>[2x]MGSSHHHHHHSSGLVPRSHMSPDLTYTEVNQNLAARENASWFSPVRFAYDW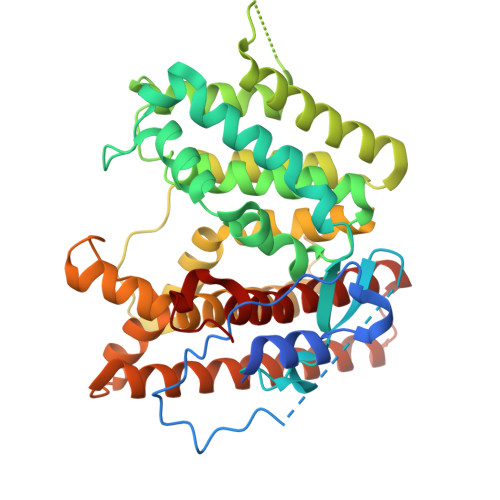LEDAPIEHLTAVPLKIRTDSPLASPKPSNVKEQSITENNENSFSISPQLTGLPWPTSFTKVRQNRHWRQSLRISTQLLELFAADDTSAQAVRRNGVSLARIASHELQTDEEDRFTKFATYIFPEANEERMKLLAATIVYIIIFDDSWEMHSEDTLGLVRDDFIRRLRGDIEGMAEHQTPLQQLINSTVQGFKDQDKTMGNGGQEVLDRLIDFCEHVPPQTKFATMGDYLSYRLIDVAFPYLLACIKFSLGSSVNVEDPKLAPILRLVSDHVSLVNDLASYDKEKRAYDNGSACYLINAVDVAQRLFSLPSAAEAKALTYSMQLLVEAQIKTELDSLVAGGILSCEELRFLDAALLMASGNVFYSVVSSRYGGKAAKLEK3,3',3'',3'''-[(7S,8S,12S,13S)-3,8,13,17-tetrakis(carboxymethyl)-8,13-dimethyl-7,8,12,13,20,24-hexahydroporphyrin-2,7,12,18-tetrayl]tetrapropanoic 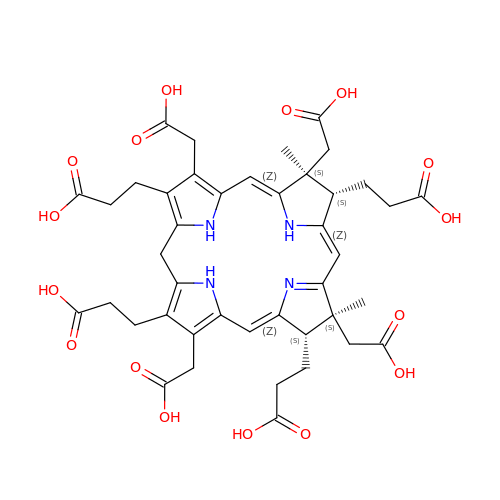acid | C42 H48 N4 O16 | CSWLXNNNLVVXKD-ORDMNHKBSA-N>HHHHHHIPTTENLYFQGAMELVNIFLETDAGRVKFAIKNTDDVCASELINKFVELLSEYIHIDQSEFYLVVKDKDIFYFKCDRGSISIVNNEFYVFDEPLLFVK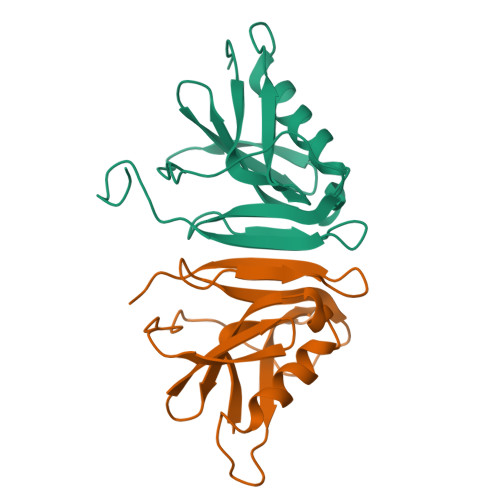DFTNVTGVEFIVTETMPCRIIPKNNHAVISVVTNHKFYNGLSL[4x]> GLIIGPEEDYDPGYFNNESDIIFQDLEKLKSHPAYLVVFLRYILSQADPGPLLFYLCSEVYQQTNPKDSRSLGKDIWNIFLEKNAPLRVKIPEMLQAEID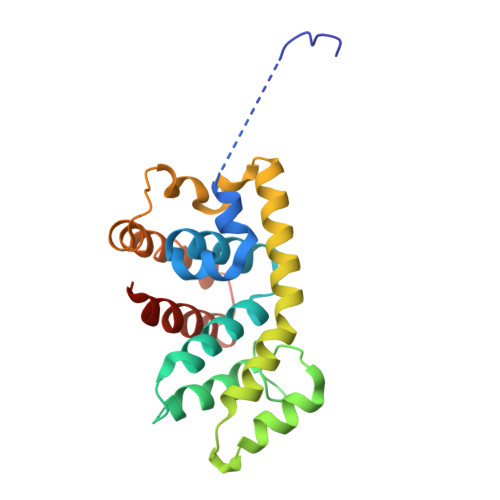LRLRNNEDPRNVLCEAQEAVMLEIQEQINDYRSKRTLGLGSLYGENDLLGLDGDPLRERQMAEKQLAALGDILSKYEEDRSAPMDFAVNTFMSHAGIRLRESR>MEADLYLDQYNFTTTAAIVSSVDRKIFVLLRDGRMLFGVLRTFDQYANLILQDCVERIYFSEENKYAEEDRGIFMIRGENVVMLGEVDIDKEDQPLEAMERIPFKEAWLTKQKNDEKRFKEETHKGKKMARHGIVYDFHKSDMY[2x];>MLFFSFFKTLVDQEVVVELKNDIEIKGTLQSVDQFLNLKLDNISSTDEKKYPHLGSVRNIFIRGSTVRYVYLNKNMVDTNLLQDATRREVMTERK[2x];>METPLDLLKLNLDERVYIKLRGARTLVGTLQAFDSHSNIVLSDAVETIYQLNNEELSESERRSEMVFIRGDTVTLISTPSEDDDGAVEI[2x];>[2x]MSGKASTEGSVTTEFLSDIIGKTVNVKLASGLLYSGRLESIDGFMNVALSSATEHYESNNNKLLNKFNSDVFLRGTQVMYISEQKI;>MSLPEILPLEVIDKTINQKVLIVLQSNREFEGTLVGFDDFVNVILEDAVEWLIDPEDESRNEKVMQHHGRMLLSGNNIAILVPGGKKTPTEAL[2x];>MHQQHSKSENKPQQQRKKFEGPKREAILDLAKYKDSKIRVKLMGGKLVIGVLKGYDQLMNLVLDDTVEYMSNPDDENNTELISKNARKLGLTVIRGTILVSLSSAEGSDVLYMQK[2x];>[2x]MKHHHHHHHGAAGTSLYKKAGENLYFQGS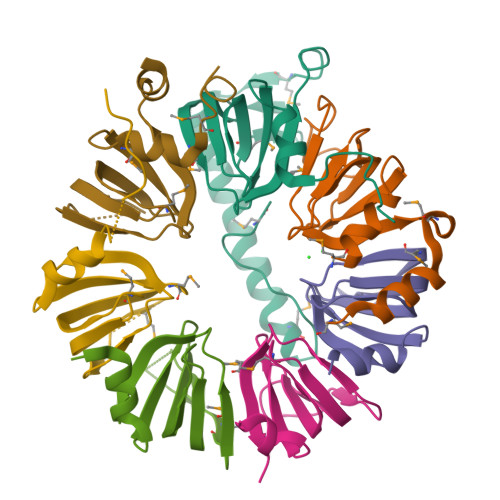MLPLYLLTNAKGQQMQIELKNGEIIQGILTNVDNWMNLTLSNVTEYSEESAINSEDNAESSKAVKLNEIYIRGTFIKFIKLQDNIIDKVKQQI> APPRLICDSRVLERYLLEAKEAEKITTGCAEHCSLNEKITVPDTKVNFYAWKRMEVGQQAVEVWQGLALLSEAVLRGQALLVKSSQPWEPLQLHVDKAVSGLRSLTTLLRALGAQKEAISPPDAASAAP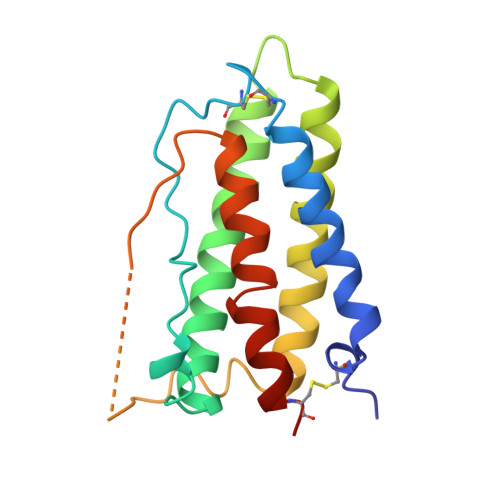LRTITADTFRKLFRVYSNFLRGKLKLYTGEACRTGDR9-AMINO-(N-(2-DIMETHYLAMINO)ETHYL)ACRIDINE-4-CARBOXAMIDE 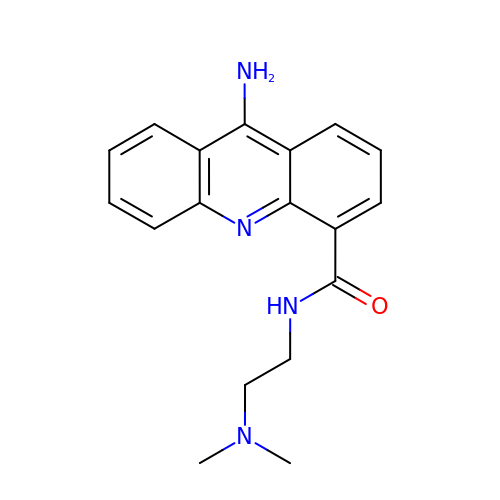| C18 H20 N4 O | YLGMVQJPGUHTRO-UHFFFAOYSA-N>MVKIYLIEHVIGAVAYDENGNIVDYITNPRDLGKITEELLNNEKGIPFSATVELLKKVNPQEVVVENEAEVPKLQALGYRVSYEPYSKVSRIFRESLPKV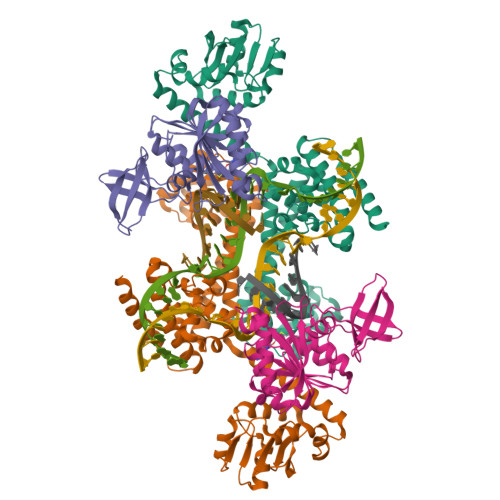AIDIKFASNEEDYYNFLHELSLEYTRRKLRSAAQKRDLLAIQAVRAMDDIDKTINLFSERLREWYSIHFPELDKLIEDHEEYATIVSRFGDRGFLTIDSLKELGFNEQRINRILDAAKKSIGADISEDDLSAMRMIANTILDLYNIRRNLNNYLEGVMKEVAPNVTALVGPALGARLLSIAGSLDELAKMPASTIQVLGAEKALFRALRSGGRPPKHGIIFQYPAIHTSPRWQRGKIARALAAKLAIAARVDAFSGRFIGDQLNEQLKKRIDEIKEKFAQHHHHHHHH[2x];>[2x]MSEVITVKQTNMENIYECEFNDGSFRLCTRNLVPNFNVYGERLIKYEGVEYREWNAFRSKLAGAILKGLKTNPIRKGTKVLYLGAASGTTISHVSDIIELNGKAYGVEFSPRVVRELLLVAQRRPNIFPLLADARFPQSYKSVVENVDVLYVDIAQPDQTDIAIYNAKFFLKVNGDMLLVIKARSIDVTKDPKEIYKTEVEKLENSNFETIQIINLDPYDKDHAIVLSKYKG>GAMCASRDDWRCARSMHEFSAKDIDGHMVNLDKYRGFVCIVTNVASQCGKTEVNYTQLVDLHARYAECGLRILAFPCNQFGKQEPGSNEEIKEFAAGYNVKFDMFSKICVNGDDAHPLWKWMKIQPKGKGILGNAIKWNFTKFLIDKNGCVVKKYGPME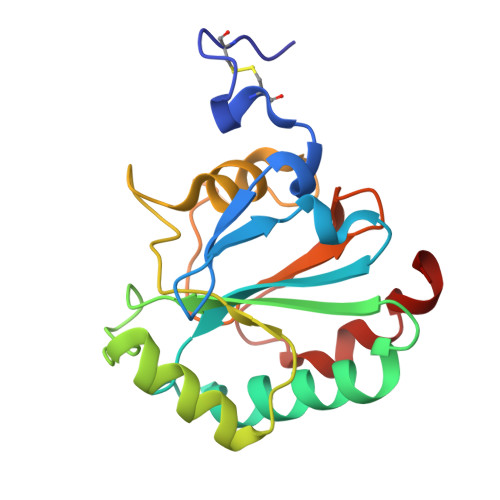EPLVIEKDLPHYF[2x]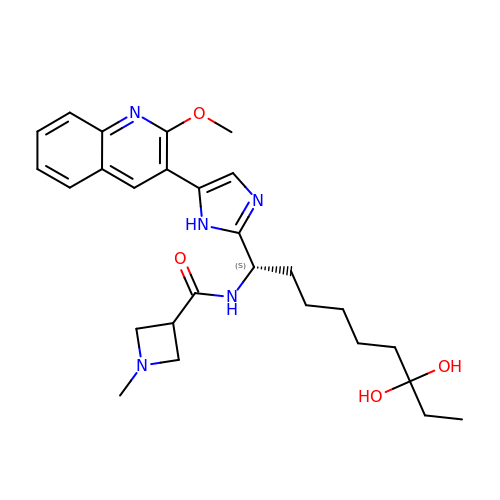N-{(1S)-7,7-dihydroxy-1-[5-(2-methoxyquinolin-3-yl)-1H-imidazol-2-yl]nonyl}-1-methylazetidine-3-carboxamide | C27 H37 N5 O4 | REZJYZJEUVOCFM-QFIPXVFZSA-N>[2x]MELWLVRHGETLWNREGRLLGWTDLPLTAEGEAQARRLKGAMPSLPAFSSDLLRARRTAELAGFSPRLYPELREIHFGALEGALWETLDPRYKEALLRFQGFHPPGGE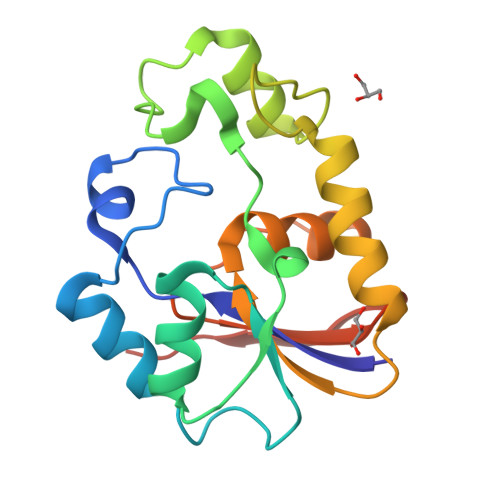SLSAFQERVFRFLEGLKAPAVLFTHGGVVRAVLRALGEDGLVPPGSAVAVDWPRRVLVRLALDGEEATG> MARENGESSSSWKKQAEDIKKIFEFKETLGTGAFSEVVLAEEKATGKLFAVKCIPKKALKGKESSIENEIAVLRKIKHENIVALEDIYESPNHLYLVMQLVSGGELFDRIVEKGFYTEKDASTLIRQVLDAVYYLHRMGIVHRDLKPENLLYYSQDEESKIMISDFGLSKMEGKGDVMSTACGTPGYVAPEVLAQKPYSKAVDCWSIGVIAYILLCGYPPFYDENDSKLFEQILKAEYEFDSPYWDDISDSAKDFIRNLMEKDPNKRYTCEQAARHPWIAGDTALNKNIHESVSAQIRKNFAKSKWRQAFNATAVVRHMRKLHLGSSLDSSNASVSSSLSLASQKDC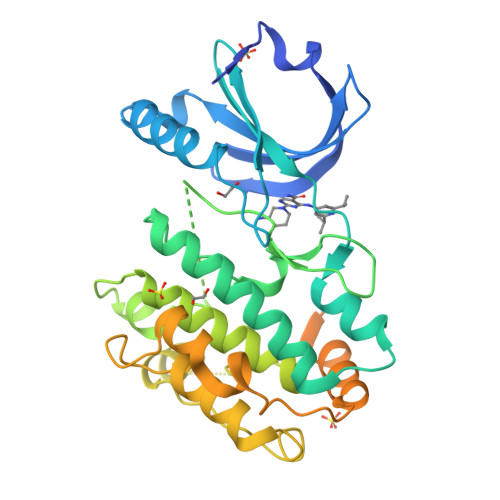LAPSTLCSFISSSSGVSGVGAERRPRPTTVTAVHSGSK>XGEIAALKQEIAALKKENAALKFEIAALKQGYY[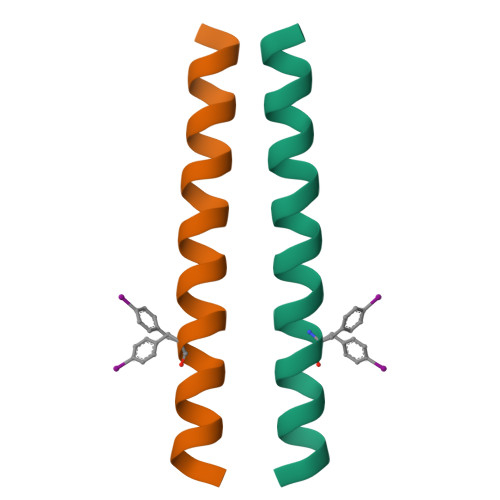2x]> GSHMNGHIYAVGGYDGSPDGSTHLNSVEAYDPERDEWHLVAPMNTRRSGVGVAVLNGHIYAVGGYDGSPDGTNHLNSVERYDPERDEWRLVAPMNTRRSGVGVAVLNGHIYAVGGYDGSPDGSTHLNSVEAYDPERDEWHLVAPMNTRRSGVGVAVLNGHIYAVGGYDGSPDGTNHLNSVERYDPERDEWRLVAPMNTRRSGVGVAVLNGHIYAVGGYDGSPDGSTHLNSVEAYDPERDEWHLVAPMNTRRSGVGVAVLNGHIYAVGGYDGSPDGTNHLNSVERYDPERDEWRLVAPMNT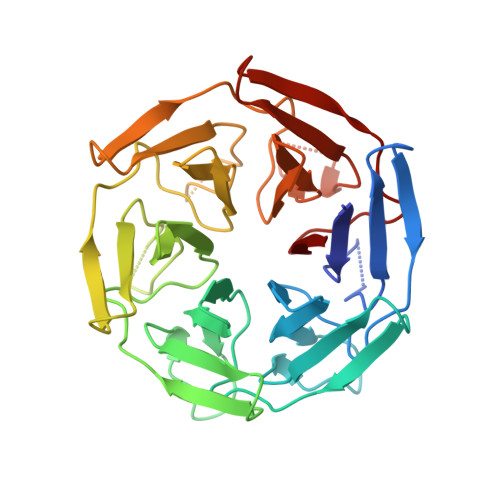RRSGVGVAVL>PQFSLWKRPVVTAYIEGQPVEVLLDTGADDSIVAGIELGNNYSPKIVGGIGGFINTKEYKNVEIEVLNKKVRATIMTGDTPINIFG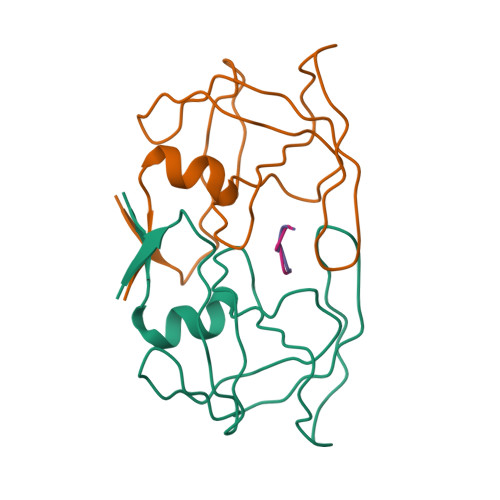RNILTALGMSLNL[4x];>[4x]FVFLEIX> GMTSFDRPFEAARPDGENPSAHETLAEGGRLRPEATYTIPARQGRAIRMAQGEALMVINRDGSQIGDFWAFVEGDCGEYLSMEHLRPTLRRVSPRPGDVLVSNRRRPILTLLEDSSPGVHDTLVASCDVHRYAQLGHEGYHDNCTDNLRMALGALGLRPTTVPCPLNLWMNTPVVEGGAMEWRPPVSRRGDHVLFRAELDVVV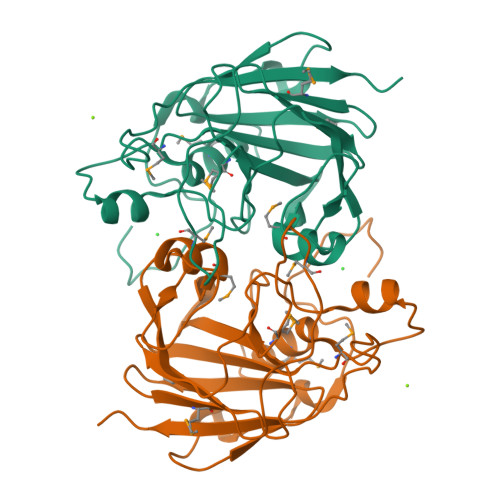VISCCPMDLLPINGEEAQPRALDVRLRPRPA> MQARKLAVDGAIEFTPRVFADDRGLLILPYQEEAFVEAHGGPLFRVAQTIHSMSKRGVVRGIHYTVTPPGTAKYVYCARGKAMDIVIDIRVGSPTFGQWDSVLMDQQDPRAVYLPVGVGHAFVALEDDTVFSYMASRSYVTQDELALSALDPALGLPIDIGVEPIVSDRDRVAITLAEAQRQGLLPDYTTSQEIERRL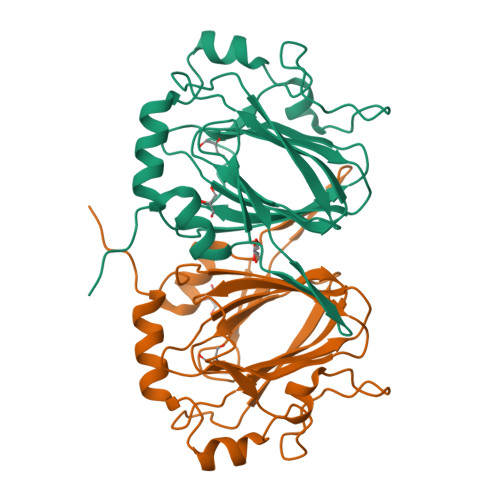TAVPVST> MKKLFLAMAVVLLSACSTFGPKDIKCEAYYMQDHVKYKANVFDRKGDMFLVSPIMAY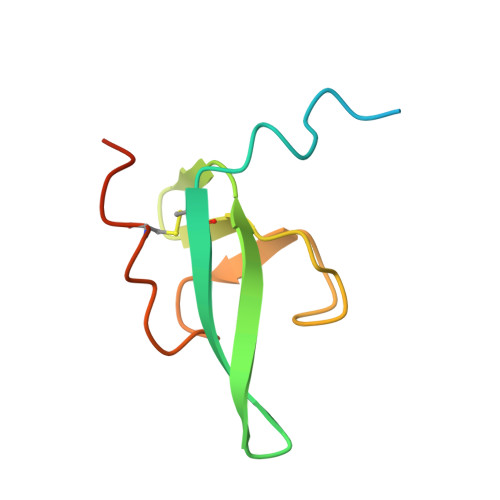GSFWAPVSYFTEGNTCEGVFHHHHHH SAS-6 organizes the rotationally ninefold symmetric cartwheel, an early assembly intermediate of centrioles that participates in establishing their symmetry and diameter. The cartwheel is organized through the homo-oligomerization of the highly conserved centriolar protein SAS-6. High-resolution crystal structures of zebrafish and C. reinhardtii SAS-6 fragments together with biochemical and biophysical characterizations demonstrated that two dimerization interfaces in SAS-6 mediate this oligomerization: a coiled-coil domain that forms a rod-like parallel dimer; and a globular N-terminal domain that forms a curved head-to-head dimer. SAS-6 is a highly conserved protein that is found in all eukaryotes that have cilia/flagella during some of their life-cycle stages.

To elucidate the structural organization of L. major SAS-6, we solved the structure of its N-terminal domain (Lm SAS-697–274) by X-ray crystallography to a resolution of 2.2 Å. The asymmetric unit (ASU) of the crystal contained three molecules that were virtually identical to each other (139 ± 2 selected pairs superpose with an rmsd of 0.70 ± 0.13 Å in secondary structure matching). Our structure demonstrates a high similarity of L. major SAS-6 to previously solved SAS-6 structures (secondary structure matching to the D. rerio SAS-6 head domain results in an rmsd of 1.59 ± 0.09 Å with 133 ± 2 selected pairs). Like these, the N-terminal domain of L. major SAS-6 consists of a 7-stranded β-barrel, capped by a helix-turn-helix motif, that forms a curved cross-handshake homo-dimer within the crystal through a highly conserved interaction interface. In this dimer, the β-hairpins formed by β-strands β6 and β7 pack antiparallelly against each other. Phenylalanine 257 at the tip of this hairpin is inserted into a conserved hydrophobic pocket that is constituted by the helix-turn-helix motif and the base of this hairpin in the B-C homo-dimer (formed by chain B and chain C in the crystal). Dimerization is also observed in solution, as judged by equilibrium ultracentrifugation, and then depends on the presence of F257. Our structural analysis also revealed the presence of an alternative arrangement of the head-to-head homo-dimer of L. major SAS-6. In the Lm SAS-697–274 crystal, the A–A homo-dimer (formed by chain A and symmetry-related chain A) shares the features of the B–C homo-dimer described above. However, in the A–A homo-dimer, the Y215 sidechain is flipped into its own hydrophobic pocket resulting in the displacement from this pocket of residue F257 of its homo-dimer partner probably weakening the interaction. We conclude that Y215 acts to partially inhibit head-to-head dimerization of L. major SAS-6.

>[3x]GPHMEAVESGVAPPPAVRTARTDLPALASPKHSAEEPQTLLETTVMVSTKMPPHEPQVRPLGVYVRTGRGGPNGVTRVVLVRLTDPTDPFFLFELELLEDDYNAFKQHLELLVDFHGFPRYLVGMLRDIADGASAYELSFVLNSAAVGDSNRGTLRVLETTDFKTVEHISLVLLRQGDAG>[2x]MPEGPELHLASQFVNEACRALVFGGCVEKSSVSRNPEVPFESSAYRISASARGKELRLILSPLPGAQPQQEPLALVFRFGMSGSFQLVPREELPRHAH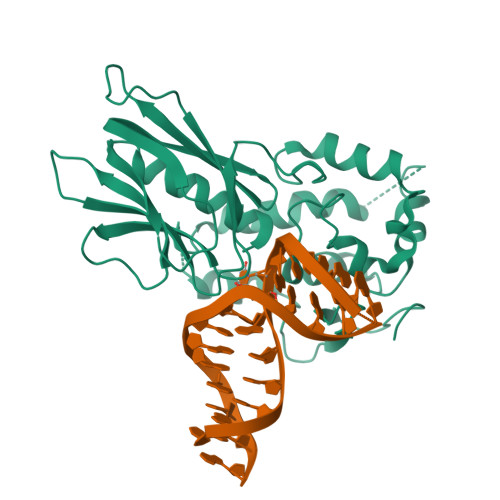LRFYTAPPGPRLALCFVDIRRFGRWDLGGKWQPGRGPCVLQEYQQFRENVLRNLADKAFDRPICEALLDQRFFNGIGNYLRAEILYRLKIPPFEKARSVLEALQQHRPSPELTLSQKIRTKLQNPDLLELCHSVPKEVVQLGGKGYGSESGEEDFAAFRAWLRCYGMPGMSSLQDRHGRTIWFQGDPGPLAPKGRKSRKKKSKATQLSPEDRVEDALPPSKAPSRTRRAKRDLPKRTATQRPEGTSLQQDPEAPTVPKKGRRKGRQAASGHCRPRKVKADIPSLEPEGTSAS;> MGEGPELHLASQFVNEACRALVFGGCVEKSSVSRNPEVPFESSAYRISASARGKELRLILSPLPGAQPQQEPLALVFRFGMSGSFQLVPREELPRHAHLRFYTAPPGPRLALCFVDIRRFGRWDLGGKWQPGRGPCVLQEYQQFRENVLRNLADKAFDRPICEALLDQRFFNGIGNYLRAEILYRLKIPPFEKARSVLEALQQHRPSPELTLSQKIRTKLQNPDLLELCHSVPKEVVQLGGRGYGSESGEEDFAAFRAWLRCYGMPGMSSLQDRHGRTIWFQGDPGPLAPKGRKSRKKKSKATQLSPEDRVEDALPPSKAPSRTRRAKRDLPKRTATQRPEGTSLQQDPEAPTVPKKGRRKGRQAASGHCRPRKVKADIPSLEPEGTSASAALGHHHHHH(1S,2R,3R,4S,5S,6R)-2,3,4,5,6-pentakis(phosphonooxy)cyclohexyl trihydrogen diphosphate | C6 H19 O27 P7 | 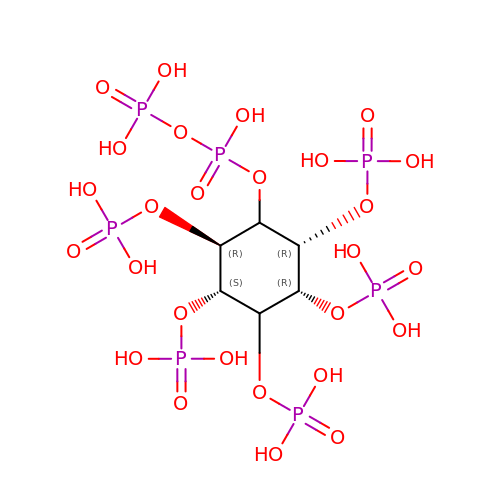UPHPWXPNZIOZJL-UOTPTPDRSA-N>MTKGKLLTTPSRLLKLVLPLSTVDHNTDRKDVAPLALLVHPQQPLSYLERLIQAELPPPDPQDSKSTTRSVTFRAMEAKDDEIKPRKKADTEGGGGSDGSVQSYSGAGREGEGKDEGEFVRWSPSTEIGDFIRDAARAKEFEVEIEGSPGVIKVAVPSFNDRTYYLRQRLRRTSRKISKLAAIKEECDKAAHRGAQRIALAGCGGLIGYWYIVYRLTFETDLGWDVMEPVTYLVGLSTLIGGYMWFLWHNREVSYRSALNITVSARQNKLYQAKGFSLQDWEGYLEEANAMRREIKAVASEYDVDWNETQDEGGDE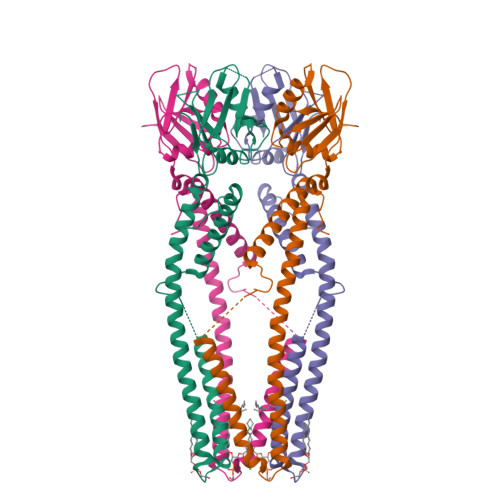KVTKALRDERKNNNGTKNKSKEGEEDDEDDGEGEEF[4x]>ADGQQGAPLNSPNTYDVTTWRIKAHPEVTAQSDIGAVINDIIADIKQRQTSPDARPGAAIIIPPGDYDLHTQVVVDVSYLTIAGFGHGFFSRSILDNSNPTGWQNLQPGASHIRVLTSPSAPQAFLVKRAGDPRLSGIVFRDFCLDGVGFTPGKNSYHNGKTGIEVASDNDSFHITGMGFVYLEHALIVRGADALRVNDNMIAECGNCVELTGAGQATIVSGNHMGAGPDGVTLLAENHEGLLVTGNNLFPRGRSLIEFTGCNRCSVTSNRLQGFYPGMLRLLNGCKENLITANHIRRTNEGYPPFIGRGNGLDDLYGVVHIAGDNNLISDNLFAYNVPPANIAPAGAQPTQILI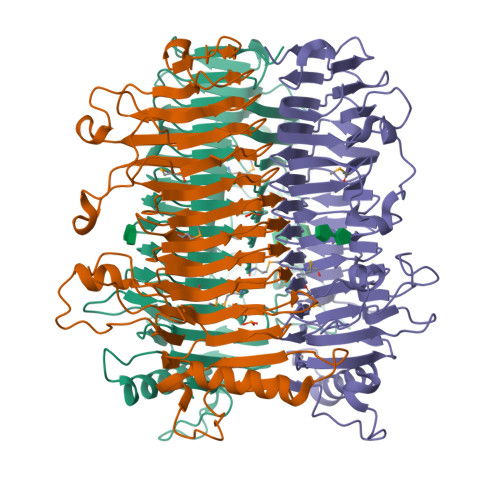AGGDANVVALNHVVSDVASQHVVLDASTTHSKVLDSGTASQITSYSSDTAIRPTP[3x]> HHHHHHFNLPPGNYKKPVLLKSTETGQYLRINPDGTVDGTRDRSDQHIQFQVSPEGGGEVLLKSTETGQYLRINPDGTVDGTRDRSDQHIQFQVSPEGGGEVLLKSTETGQYLRINPDGTVDGTRDRSDQHIQF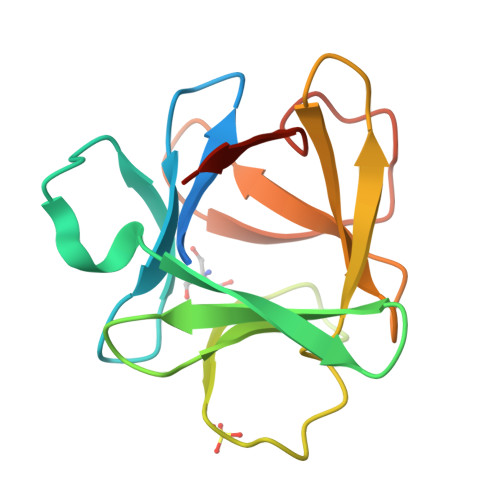QVSPEGGG4-(2-amino-5-chloro-1H-benzimidazol-1-yl)-N-cyclohexyl-N-methylbutanamide | C18 H25 Cl N4 O | 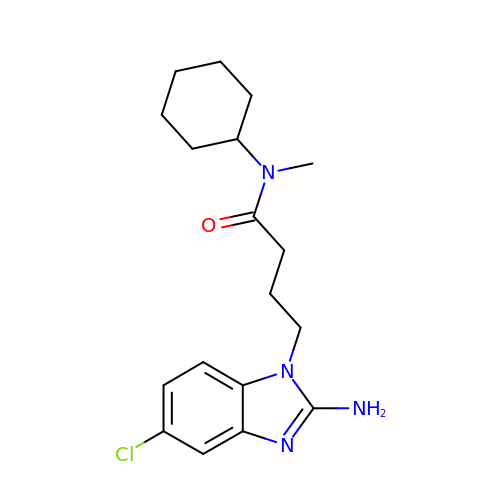UIWHCBCBZBYNDS-UHFFFAOYSA-N> ATITQDTPINQIFTDTALAEKMKTVLGKTNVTDTVSQTDLDQVTTLQADRLGIKSIDGVEYLNNLTQINFSNNQLTDITPLKNLTKLVDILMNNNQIADITPLANLTNLTGLTLFNNQITDIDPLKNLTNLNRLELSSNTISDISALSGLTSLQQLSFSSNQVTDLKPLANLTTLERLDISSNKVSDISVLAKLTNLESLIATNNQISDITPLGILTNLDELSLNGNQLKDIGTLASLTNLTDLDLANNQISNLAPLSGLTKLTELKLGANQISNISPLAGLTALTN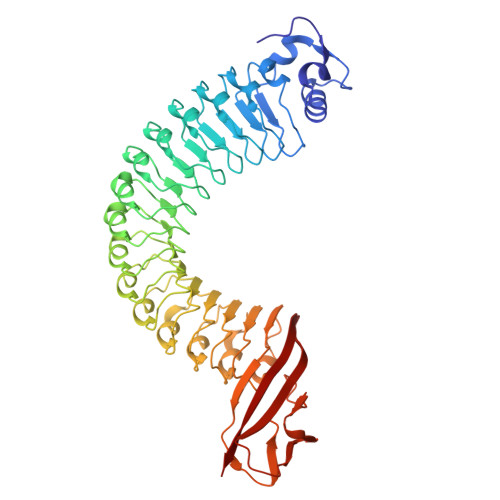LELNENQLEDISPISNLKNLTYLTLYFNNISDISPVSSLTKLQRLFFSNNKVSDVSSLANLTNINWLSAGHNQISDLTPLANLTRITQLGLNDQAWTNAPVNYKANVSIPNTVKNVTGALIAPATISDGGSYTEPDITWNLPSYTNEVSYTFSQPVTIGKGTTTFSGTVTQPLKA> 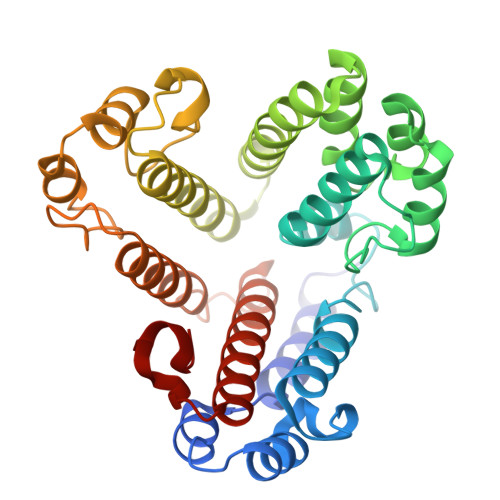DDFAYLNARVRVRRGTLLKESFFQEALDLSFADFLRLLSETVYGGELAGQGLPDVDRAVLRTQAKLVGDLPRLVTGEAREAVRLLLLRNDLHNLQALLRAKATGRPFEEVLLLPGTLREEVWRQAYEAQDPAGMAQVLAVPGHPLARALRAVLRETQDLARVEALLAKRFFEDVAKAAKGLDQPALRDYLALEVDAENLRTAFKLQGSGLAPDAFFLKGGRFVDRVRFARLMEGDYAVLDELSGTPFSGLSGVRDLKALERGLRCVLLKEAKKGVQDPLGVGLVLAYVKEREWEAVRLRLLARRAYFGLPRAQVEEEVVC>[8x]GPSGRNSSLSSVSGSTVAGDKIPIKTTHAALSWNSLKIGKSEIKEFTIRNTSNNKIKIQATISDSEKNFRFLRERETIGTTIVLALQGSESRTLSVVFSPHHIGAASGKIIFRHYQSKKEDSESLPSRQIFLYGYGGYSKVEISEVFKDT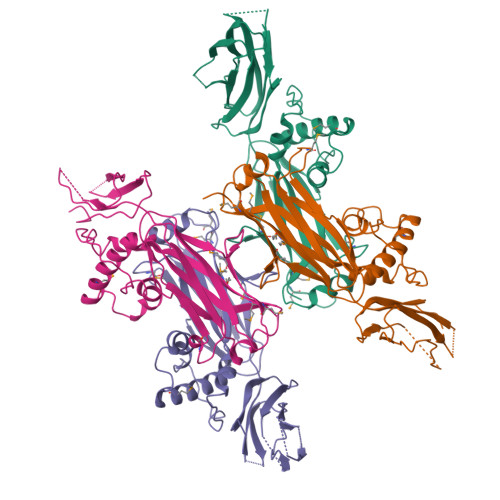NGKMWLSFGMLNSENSLNAKIKLQNTGDLCSYVKIKLTPKAVYPTMISSWQVNPTELLLNPKEVQWVTLEFHPRKEDLALLQKSDVSHVGTLLITHGDEPTRLRIRRLYKKMKETGELNGNENETFRNIVHPICKVFSGEQLVSDVIPIRDSVQNFGDLCREIRQHEIMLTMEVCADETLTVLHDNPDESQ> YGGGSSGGGS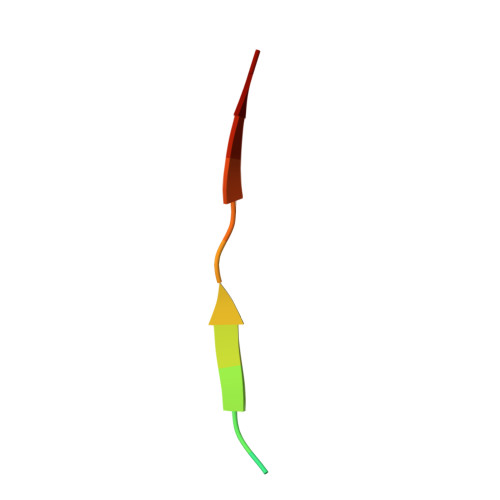SGGGH>DNDDYDEKPREECGVVGIYGDSEASRLCYLALHALQHRGQEGAGIVTVSKDKVLQTITGVGLVSEVFSESKLDQLPGDIAIGHVRYSTAGSSMLKNVQPFVAGYRFGSVGVAHNGNLVNYTKLRADLEENGSIFNTSSDTEVVLHLIAISKARPFFMRIVDACEKLQGAYSMVFVTEDKLVAVRDPHGFRPLVMGRRSNGAVVFASETCALDLIEATYEREVYPGEVLVVDKDGVKCQCLMPHPEPKQCIFEHIYFSLPNSIVFGRSVYESRHVFGEILATESPVDCDVVIAVPDSGVVAALGYAAKAGVAFQQGLIRSHYVGRTFIEPSQKIRDFGVKLKLSPVRGVLEGKRVVVVDDSIVRGTTSSKIVRLLREAGAKEVHMRIASPPIIASCYYGVDTPSSNELISNRMSVDEIRDYIGCDSLAFLSFETLKKHLGEDSRSFCYACFTGDYPVKPTEDKVKRGGDFIDDGLVGGIHNIEGGWVR[2x]

GPRATase catalyzes the first committed step of purine biosynthesis, transforming phosphoribosylpyrophosphate (PRPP) to phosphoribosylamine (PRA) with amide group of glutamine as nitrogen source. The reaction catalyzed by GPRATases is carried out as two half-reactions by two separate domains, in tight allosteric communication between each other. One is the Glnase domain where Gln is hydrolyzed to yield ammonia. And then, the ammonia is transferred through a ~20-Å hydrophobic channel to a distal PRTase domain, in which PRA is synthesized from PRPP and ammonia.

We solved the crystal structure of a recombinant AtGPRAT275-561 without the predicted chloroplast transit peptide at 3.07 Å resolution. The crystal belonged to the P3121 space group and two AtGPRAT2 molecules were found in the asymmetric unit, each with a 4Fe-4S cofactor. However, the PISA (Proteins, Interfaces, Structures and Assemblies) server indicated that AtGPRAT2 exists as a homo-tetramer in crystal as other members of this family. Consistent with this, in the AtGPRAT2 structure, the first residue with interpretable electron density was the predicted N-terminal Cys87, the mutation of which abolished the activity of the enzyme. Similar to members of this family, the overall structure of AtGPRAT2 folds into an N-terminal glutaminase (Glnase) domain (residues 87-320) and a C-terminal phosphoribosyltransferase (PRTase) domain (residues 321-546). Structural comparison indicated that AtGPRAT2 adopts an inactive, open conformation as compared to the structures of the EcGPRAT in the presence or absence of the PRPP analog carboxylic PRPP (cPRPP), which represent the active and inactive state, respectively. In contrary to the glutamine loop of EcGPRAT, which is in a closed conformation no matter glutamine binds or not, the glutamine loop of AtGPRAT2 exhibits an open conformation more similar to that of BsGPRAT. Nevertheless, the glutamine loop of AtGPRAT2 opens to an extent larger than that of BsGPRAT, and forms a 310 helix. The PRTase flexible loops of AtGPRAT and bacterial enzymes display different open conformations, consistent with the disordered feature of this loop. However, similar as BsGPRAT, AtGPRAT2 does not contain the helix and the corresponding region folds as a flexible loop.>[2x]MNMFFRLTALAGLLAIAGQTFAVEDITRADQIPVLKEETQHATVSERVTSRFTRSHYRQFDLDQAFSAKIFDRYLNLLDYSHNVLLASDVEQFAKKKTELGDELRSGKLDVFYDLYNLAQKRRFERYQYALSVLEKPMDFTGNDTYNLDRSKAPWPKNEAELNALWDSKVKFDELSLKLTGKTDKEIRETLTRRYK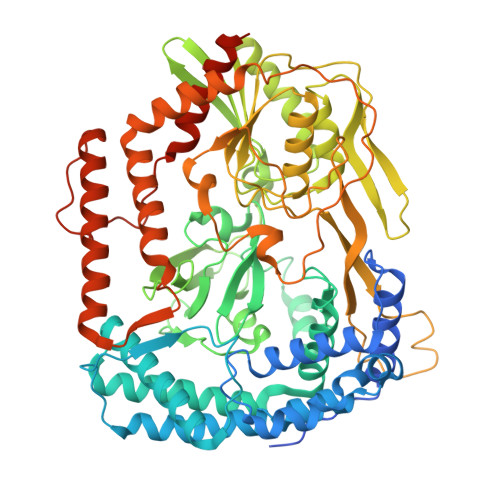FAIRRLAQTNSEDVFSLAMTAFAREIDPHTNYLSPRNTEQFNTEMSLSLEGIGAVYQMDDDYTVINSMVAGGPAAKSKAISVGDKIVGVGQTGKPMVDVIGWRLDDVVALIKGPKGSKVRLEILPAGKGTKTRTVTLTRERIRLEDRAVKMSVKTVGKEKVGVLDIPGFYVGLTDDVKVQLQKLEKQNVSSVIIDLRSNGGGALTEAVSLSGLFIPAGPIVQVRDNNGKVREDSDTDGQVFYKGPLVVLVDRFSAIASEIFAAAMQDYGRALVVGEPTFGKGTVQQYRSLNRIYDQMLRPEWPALGSVQYTIQKFYRVNGGSTQRKGVTPDIIMPTGNEETETGEKFEDNALPWDSIDAATYVKSGDLTAFEPELLKEHNARIAKDPEFQNIMKDIARFNAMKDKRNIVSLNYAVREKENNEDDATRLARLNERFKREGKPELKKLDDLPKDYQEPDPYLDETVNIALDLAKLEKARPAEQPAPVKHHHHHH>RRGLLPNHIWQGDVTHYKYKKYKYCLHVWVDTFSGAVSVSCKKKETSCETISAFLQAISLLGKPLHINTDNGPAFLSQEFQEFCTSYHIKHSTHIPYNPTSSGLVERTNGIIKNLLNKYLLDCPNLPLDNAINKALWTLNQLNVMNP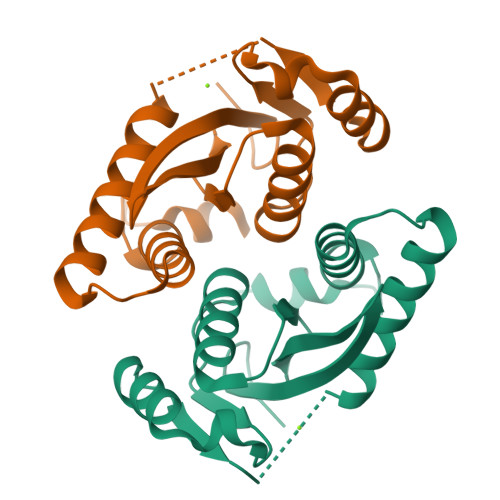SGKTRWQIHHSPPLPPI[4x]>[2x]STTATEGHKPVPCGWERVVKQRLSGKTAGK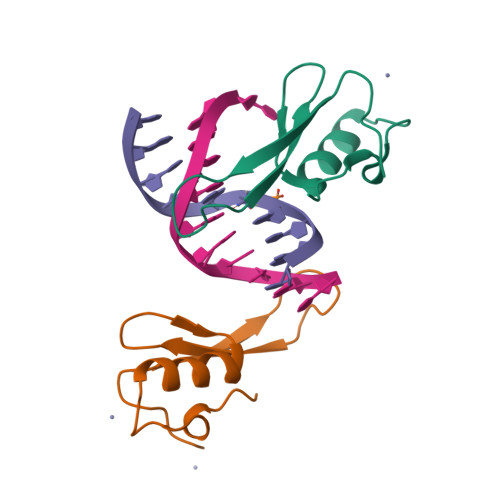FDVYFISPQGLKFRSKRSLANYLLKNGETFLKPEDFNFTVLPKG> MTTKKFDEADKSNVEMYLIQAGVKQDAAATMGIWTAQELHRIKSQSYEEDYPVGSALRVFPVTTELSPTDKTFEYMTFDKVGTAQIIADYTDDLPLVDALGTSEFGKVFRLGNAYLISIDEIKAGQATGRPLSTRKASACQLAHDQLVNRLVFKGSAPHKIVSVFNHPNITKITSGKWIDVSTMKPETAEAELTQAIETIETITRGQHRATNILIPPSMRKVLAIRMPETTMSYLDYFKSQ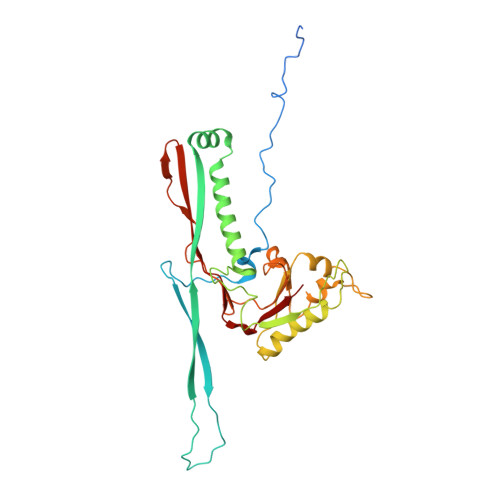NSGIEIDSIAELEDIDGAGTKGVLVYEKNPMNMSIEIPEAFNMLPAQPKDLHFKVPCTSKCTGLTIYRPMTIVLITGV>MKHTELRAAVLDALEKHDTGATFFDGRPAVFDEADFPAVAVYLTGAEYTGEELDSDTWQAELHIEVFLPAQVPDSELDAWMESRIYPVMSDIPALSDLITSMVASGYDYRRDDDAGLWSSADLTYVITYEM[6x];>[6x]MPVPNPTMPVKGAGTTLWVYKGSGDPYANPLSDVDWSRLAKVKDLTPGELTAESYDDSYLDDEDADWTATGQGQKSAGDTSFTLAWMPGEQGQQALLAWFNEGDTRAYKIRFPNGTVDVFRGWVSSIGKAVTAKEVITRTVKVTNVGRPSMAEDRSTVTAATGMTVTPASTSVVKGQSTTLTVAFQPEGVTDKSFRAVSADKTKATVSVSGMTITVNGVAAGKVNIPVVSGNGEFAAVAEITVTAS;>MADFDNLFDAAIARADETIRGYMGTSATITSGEQSGAVIRGVFDDPENISYAGQGVRVEGSSPSLFVRTDEVRQLRRGDTLTIGEENFWVDRVSPDDGGSCHLWLGRGVPPAVNRRR[6x]

The temperate phage lambda, which infects the bacterium Escherichia coli, belongs to Siphoviridae. The virion of the lambda phage comprises an icosahedral head and a long flexible tail. The tail, which comprises the tail tube and tail tip, connects with the head through the neck. The neck–tail complex comprises a channel formed by stacked 12-fold and hexameric rings and a 3-fold symmetrical tip.

Six copies of the stopper protein gpFII are assembled into a hexameric ring connecting the adaptor. The gpFII structure comprises 4 domains: an N-terminal α-helix (residues 4–24), a β-sandwich (residues 25–41 and 63–107), a β-hairpin (residues 46–62) inserted in the β-sandwich, and a C-terminal loop (residues 108–117). A comparison of our gpFII structure with the NMR structure of gpFII monomer in solution revealed that the structure of gpFII monomer in solution undergoes notable conformational changes to reach the assembled state. The N-terminal loop becomes the α-helix domain. In addition, the stopper ring (gpFII) of the lambda structure exhibits an open conformation. The tail tube connects with the neck via interaction between the ring of the stopper protein gpFII and that of the tail terminal protein gpU. All 131 residues of gpU comprise an antiparallel five-strand β-sheet flanked by 2 α-helices, with an O-shaped loop (O-loop, residues 25–37) inserted between β1 and β2 and an extended-loop (E-loop, residues 45–58) inserted between β2 and β3. To adapt to ring–ring interactions, the long loop (residues 46–62) observed in the structure of gpFII monomer in solution becomes a β-hairpin, which inserts into the inner surface of the gpU ring and interacts with the O-loop of gpU through β-sheet augmentation. The E-loop of gpU provides an attachment site for the major tail protein gpV through electrostatic interactions. The surface of the gpU ring is strongly negatively charged, probably facilitating the correct positioning of the packaged DNA.>MKLARFLAKGRVHQGVYREGLLLDEAGEAHRPEDVTWLLPFTPGKILGVALNYADHAEELGLSRPEEPALFWKPNTSLLPHKGVVLYPKGARFVHYEVELAVVVGRPMKRVRAKDALDYVLGYTIANDLVARDYVTNTFRPPIRAKGRDTFLPLGPFLVVEEVEDPQDLWLRAYVNGELRQEGHTSRMLYSVAELLEFISEFMTLEPYDVLLTGTPKGISQVRPGDV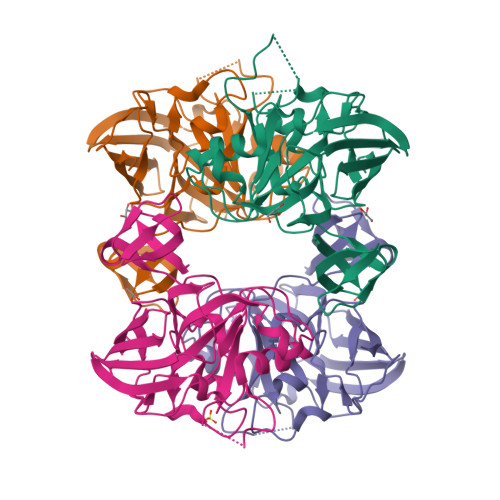MRLEIEGLGALENPIEEEP[4x]The transactive response DNA-binding protein-43 (TDP-43) is a multi-facet protein involved in phase separation, RNA-binding, and alternative splicing. In the context of neurodegenerative diseases, abnormal aggregation of TDP-43 has been linked to amyotrophic lateral sclerosis and frontotemporal lobar degeneration through the aggregation of its C-terminal domain. Here, we report a cryo-electron microscopy (cryo-EM)-based structural characterization of TDP-43 fibrils obtained from the full-length protein. We found three different fibril structures in our sample that share the same basic fibril protein fold and differ in the number and relative arrangement of the fibril protofilaments.

Morphology-2 show a width of 10.4 ± 0.6 nm (n = 50), while the fibril cross-overs are hardly visible and no crossover distance could be measured. Approximately 59% of the fibrils visible in the sample correspond to Morphology-1 and 17% to Morphology-2. The 3D maps reached spatial resolutions of 3.76 Å (Morphology-1a) and 4.05 Å (Morphology-1b), based on the 0.143 Fourier Shell Correlation (FSC) criterion. In the case of Morphology-2, it was not possible to identify more than one 3D class, and the 3D map of this fibril structure was refined to a resolution of 3.86 Å. Morphology-2, finally, contains three structurally equal, in-register fibril protein stacks, and the fibril is C3-symmetrical. Despite these differences, we find the interfaces between the adjacent protein stacks to be formed by the same two amino acid residues (Met311 and Phe313) in the three fibrils. The three fibril structures contain essentially the same fibril protein conformation that is formed by 45 residues (Gly304 to Gly348) from the LC domain. All fibril proteins contain arch that is formed by residues Ala328-Ala341, while residues Gly304-Ala326 are wrapped around this arch.

>MSEYIRVTEDENDEPIEIPSEDDGTVLLSTVTAQFPGACGLRYRNPVSQCMRGVRLVEGILHAPDAGWGNLVYVVNYPKDNKRKMDETDASSAVKVKRAVQKTSDLIVLGLPWKTTEQDLKEYFSTFGEVLMVQVKKDLKTGHSKGFGFVRFTEYETQVKVMSQRHMIDGRWCDCKLPNSKQSQDEPLRSRKVFVGRCTEDMTEDELREFFSQYGDVMDVFIPKPFRAFAFVTFADDQIAQSLCGEDLIIKGISVHISNAEPKHNSNRQLERSGRFGGNPGGFGNQGGFGNSRGGGAGLGNNQGSNMGGGMNFGAFSINPAMMAAAQAALQSSWGMMGMLASQQNQSGPSGNNQNQGNMQREPNQAFGSGNNSYSGSNSGAAIGWGSASNAGSGSGFNGGFGSSMDSKSSGWGM[18x]>MFTGSIVAIVTPMDEKGNVCRASLKKLIDYHVASGTSAIVSVGTTGESATLNHDEHADVVMMTLDLADGRIPVIAGTGANATAEAISLTQRFNDSGIVGCLTVTPYYNRPSQEGLYQHFKAIAEHTDLPQILYNVPSATGCDLLPETVGRLAKVKNIIGIKEATGNLTRVNQIKELVSDDFVLLSGDDASALDFMQLGGHGVISVTANVAARDMAQMCKLAAEGHFAEARVINQRLMPLHNKLFVEPNPIPVKWACKELGLVATDTLRLPMTPITDSGRETVRAALKH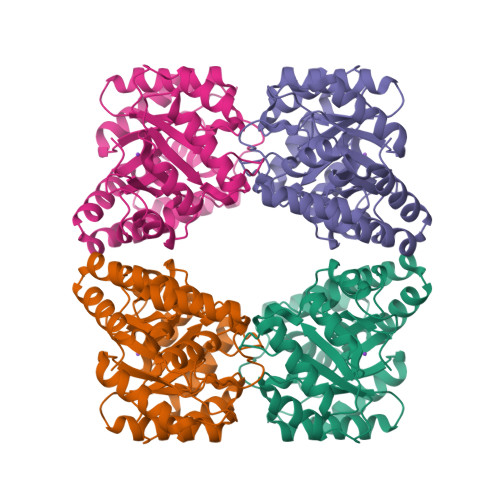AGLL[2x]> MSFDPNTQGFSTASIHAGYEPDDYYGSINTPIYASTTFAQNAPNELRKGYEYTRVGNPTIVALEQTVAALEGAKYGRAFSSGMAATDILFRIILKPGDHIVLGNDAYGGTYRLIDTVFTAWGVEYTVVDTSVVEEVKAAIKDNTKLIWVETPTNPALGITDIEAVAKLTEGTNAKLVVDNTFASPYLQQPLKLGAHAVLHSTTKYIGGHSDVVGGLVVTNDQEMDEELLFMQGGIGPIPSVFDAYLTARGLKTLAVRMDRHCDNAEKIAEFLDSRPEVSTVLYPGLKNHPGHEVAAKQMK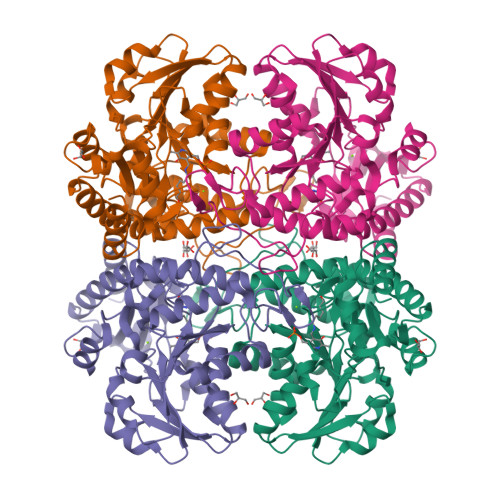RFGGMISVRFAGGEEAAKKFCTSTKLICLAESLGGVESLLEHPATMTHQSAAGSQLEVPRDLVRISIGIEDIEDLLADVEQALNNLHHHHHH We describe here the use of an artificial cofactor employing the well‐known biotin‐streptavidin system to catalyze a Baylis‐Hillman reaction. As protein host, we chose streptavidin, as it can be easily crystallized and thereby supports the design process. There are several examples using streptavidin as the host for these cofactors, since its natural ligand biotin binds strongly (K d∼10−15 M) and is easy to modify with catalysts at the carboxylic acid group. No enzyme is known to naturally catalyze the Baylis‐Hillman reaction, a very versatile and atom‐economic C−C bond forming reaction for the production of various functionalized compounds and intermediates of active pharmaceutical ingredients (APIs).

We chose a derivative of DMAP as the artificial cofactor due to its low steric demand, which will facilitate its inclusion into the protein scaffold. The protein host around the cofactor was rationally designed on the basis of high‐resolution crystal structures obtained after each variation of the amino acid sequence. The location of the catalyst is in a shallow cavity at the surface of the protein. The system was evolved through repeated cycles of mutagenesis, activity tests, and structure determination. According to the presented structures and calculations the catalytically active site is too shallow to undergo interactions with 1.

>MASMTGGQQMGRDEAGITGTWYNQLGSTFIVTAGADGALTGTYESAAGKAESRYVLTGRYDSAPATDGSGTALGWTVAWKNNYRNAHSATTWSGQYVGGAEARINTQWLLTSGATEANGWASTLVGHDTFTKVKPSAASIDAAKKAGVNNGNPLDAVQQ[2x]> MASAHIALELDKTKVKVGDVIVATVKAKNMTSMAGIQVNIKYDPEVLQAIDPATGKPFTKETLLVDPELLSNREYNPLLTAVNDINSGIINYASCYVYWDSYRESGVSESTGIIGKVGFKVLKAANTTVKLEETRFTPNSIDGTLVIDWYGQQIVGYKVIQPDLEHHHHHH;> MNNDSTDKTTVSGYISVDFDYPPESESKIKSGFNVKVAGTELSTKTDEKGYFEISGIPGDMREFTLEISKRNYLKRNVTVNGTGKLVVSTEDNPLILWAGDVERKGVQDNAINMVDVMEISKVFGTRAGDEEYVAELDLNMDGAINLFDIAIVIRHFNALPSRY

In addition, cellulosomes are central elements for the production of readily available sugars in the gastrointestinal tract of a variety of mammals4. It is now well established that a wide array of highly ordered protein-protein interactions involving dockerin and cohesin modules (defined herein as Doc and Coh, respectively) mediate both cellulosome assembly and cellulosome cell-surface attachment. Primary scaffoldins, in addition to containing multiple type-I Cohs, have a divergent type-II Doc that binds to type-II Cohs located in cell-surface anchoring scaffoldins, providing a mechanism to tether the cellulosome to the bacterial cell envelope. In addition to ScaA, inspection of C. thermocellum genome revealed the presence of an ORF (Cthe_1806) encoding a protein comprising 2177 amino acids and containing a putative type-II Doc, which was termed CipB. Type-II Docs of primary scaffoldins ScaA and CipB in C. thermocellum possess two distinct Coh-binding surfaces that recognize different Coh partners.

ScaC2 Coh was selected, as both ScaA and CipB Docs were shown to bind preferentially to this Coh. In the complex, the ScaC2 Coh formed a typical flattened, elongated 9-stranded β-barrel with a jelly-roll topology. The XDoc dyad was modelled as one single polypeptide chain of 164 amino acids with the first 98 corresponding to the X-module and the remaining to the type-II Doc. The CipB type-II Doc (residues 99–164) formed two loop-helix F-hand motifs separated by a 23-residue linker that also forms a small helix. Both F-hand motif loops coordinated a calcium ion in a typical octahedral geometry. In the CtCohScaC2-XDocCipB complex the X-module stabilized both Doc calcium binding loops, while in the ScaA Coh-XDoc complex the X-module only interacted with the first calcium-binding loop of the Doc. Similar to what was observed in the CtCohScaF-XDocScaA complex, both helices of CipB Doc interacted with the planar surface of the ScaC2 Coh comprising β-strands 8-3-6-5. Similar to what was observed in the CtCohScaF-XDocScaA complex, the C-terminal helix (helix 3) of CipB Doc dominated Coh recognition. In addition, the CohScaC2-XDocCipB interacting region is predominantly hydrophobic. Only two direct hydrogen bonds were identified at the ScaC2 Coh:CipB XDoc interface: Nδ2 of Asn146 Doc and O of Phe136 Coh, and N of Leu147 Doc and Oε1 of Gln37 Coh.> GKLLLEG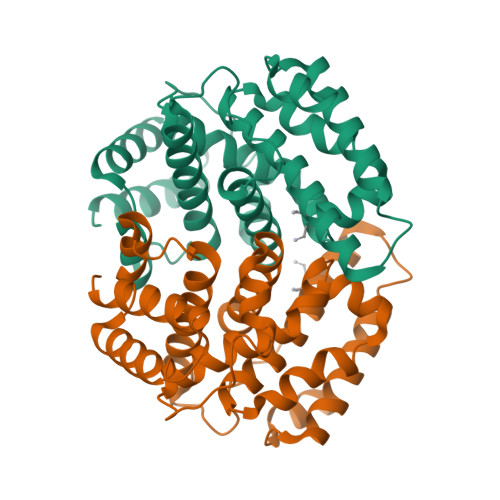VKEQDPVDKFTYLLLQPLTEATLSDAVNFIVEKYSAELPDEGDASLVVRSQLGCQFFFLVTRTLAHDQRELAKLVQTLIPRPVRLEVFPGLQRSVFKSSVFLGHHIIQIFMGAKKPFQDWSFVGLAQDFECPWRRLAIAELLKKFSVSVVEKVFDNPVALIPQHESDNEALIELVTNALRFALWIVEFYETETNEKSIKELAFLDHSSKTLLIESFTKFLQGKDVKDQDHLKRIIDALEKS[(2-{[2-(6-oxo-1,6-dihydro-9H-purin-9-yl)ethyl](2-phosphonoethyl)amino}ethoxy)methyl]phosphonic 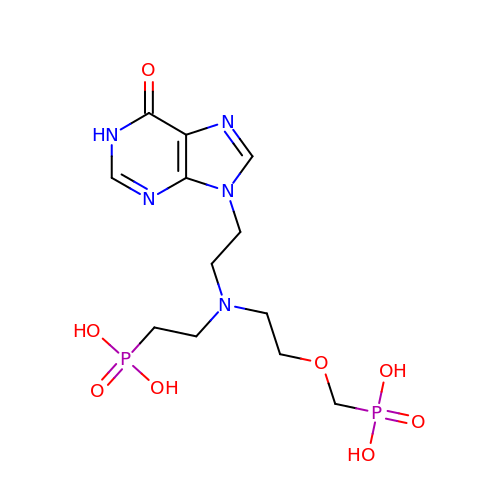acid | C12 H21 N5 O8 P2 | DOQZRNUAQKXUPD-UHFFFAOYSA-N>GSMASSDTEGKRVVVIGGGLVGALNACFLAKRNFQVDVYEAREDIRVANFMRGRSINLALSYRGRQALKAVGLEDQIVSKGVPMKARMIHSLSGKKSAIPYGNKSQYILSISREKLNKDLLTAVESYPNAKVHFGHKLSKCCPEEGILTMLGPNKVPRDITCDLIVGCDGAYSTVRAHLMKKPRFDYSQQYIPHGYMELTIPPKNGEYAMEPNCLHIWPRNAFMMIALPNMDKSFTCTLFMSFEEFEKLPTHSDVLDFFQKNFPDAIPLMGEQALMRDFFLLPAQPMISVKCSPFHLKSRCVLMGDA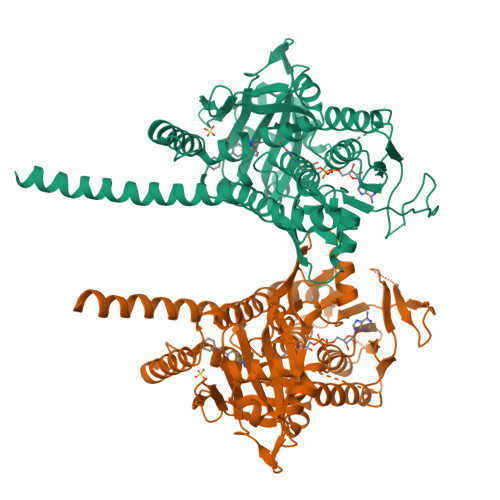AHAIVPFFGQGMNAGFEDCLVFDELMDKFNNDLSVCLPEFSRFRIPDDHAISDLSMYNYIEMRAHVNSRWFLFQRLLDKFLHALMPSTFIPLYTMVAFTRIRYHEAVLRWHWQKKVINRGLFVLGSLVAIGSAYILVHHLSPRPLELLRSAWTGTSGHWNRSADISPRVPWSHENLYFQGDYKDDDDK[2x]>[2x]EXCQKWMWTCDSARACCEG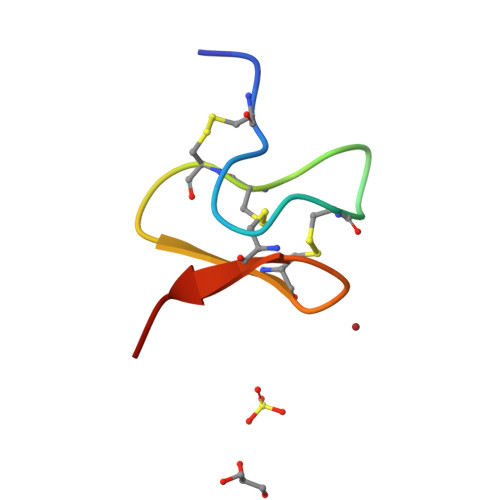LRCKLWCRKEIX1-[2-(3-{[(2,4-diamino-6-ethylpyrimidin-5-yl)oxy]methyl}azetidin-1-yl)phenyl]piperidine-4-carboxylic 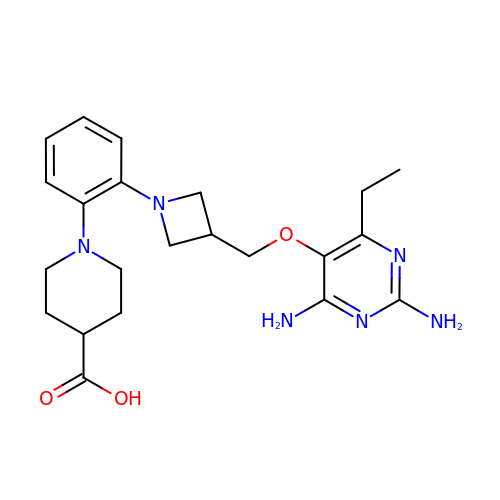acid | C22 H30 N6 O3 | HUNFOZYRLCOIAK-UHFFFAOYSA-N(2R)-2-[(2-amino-7-fluoropyrido[3,2-d]pyrimidin-4-yl)amino]-2-methylhexan-1-ol | C14 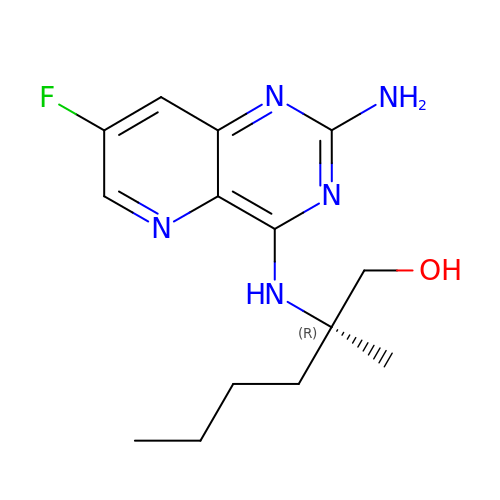H20 F N5 O | HTCJUBZBSJQWBW-CQSZACIVSA-N>EELPQIEIVQEGDNTTFAKPGDTVTIHYDGKLTNGKEFDSSRKRGKPFTCTVGVGQVIKGWDISLTNNYGKGGA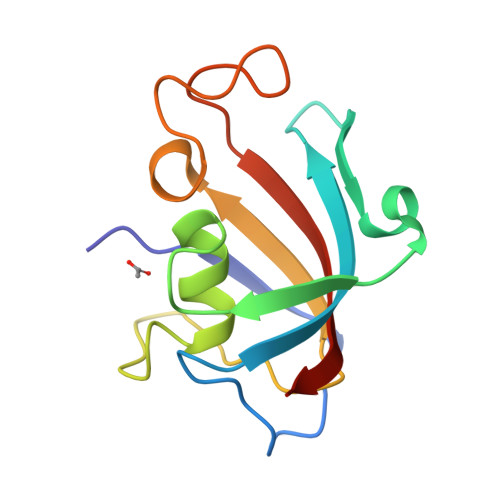NLPKISKGTKAILTIPPNLAYGPRGIPPIIGPNETLVFEVELLGVNGQ[2x]3-[(5S)-1-ACETYL-3-(2-CHLOROPHENYL)-4,5-DIHYDRO-1H-PYRAZOL-5-YL]PHENOL | C17 H15 Cl N2 O2 | 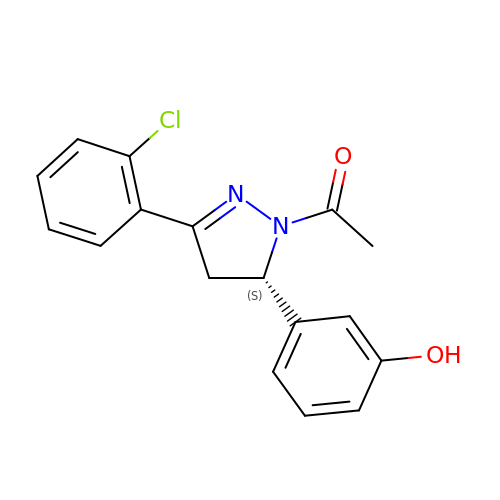QBZAPFWYAPXRGQ-KRWDZBQOSA-N Here we investigated a protein containing a CARF domain fused Toll/interleukin-1 receptor (TIR) domain, Cat1. We found that Cat1 provides immunity by cleaving and depleting NAD+ molecules from the infected host, inducing a growth arrest that prevents viral propagation. Cat1 forms dimers that stack upon each other to generate long filaments that are maintained by bound cOA ligands, with stacked TIR domains forming the NAD+ cleavage catalytic sites. Further, Cat1 filaments assemble into unique trigonal and pentagonal networks that enhance NAD+ degradation.

To understand the effects of Cat1 filamentation on the catalysis of NAD+ cleavage at the atomic level, we solved cryo-EM structures of cA4-bound Cat1 in the presence of a non-hydrolysable NAD+ analogue, benzamide adenine dinucleotide (BAD) or NAD+ at 3.3 Å and 4 Å resolution, respectively. We could resolve similar pentameric filament network formation for class 1 that represented the largest number of particles for both cA4-BAD-Cat1-His6 and cA4-NAD+-Cat1-His6 and therefore these were processed further, to the exclusion of other classes in both complexes that were part of the same network. We modelled a pair of Cat1 dimers in the map for each structure. In the case of the cA4− NAD+-Cat1-His6 structure, the observed density was sufficient to model ADPR, but neither the NAD+ substrate nor the other reaction product, NAM. In both cases we observed that residues S7, H8, N9, N10, D33, S68 and E74 from one TIR domain, and K121 and Y122 from the other, line the NADase active site. The BB-loop is predicted to control the access to the NADase active site in other TIR proteins. Both structures revealed that the active site is formed by two TIR domains from a pair of stacked Cat1 dimeric repeat units, suggesting that the catalytic activity relies on the multimerization of Cat1 dimers upon cA4 signal recognition. We tested the importance of these residues for Cat1 activity by making alanine substitutions (N10A, D33A, S68A, E74A, K121A and Y122A). The mutants were tested in vivo by measuring their toxicity during the type III-A CRISPR-Cas response and were all found to be defective in causing a growth arrest in staphylococci. While the D33A substitution reduced activity only partially, the Y122A mutation completely abrogated NAD+ cleavage. Altogether these data showed that Cat1 active site is formed through the interaction of two stacked TIR domains from different dimers, a finding that provides an explanation for the importance of filamentation for its enzymatic activity, as well as for the cooperativity of NAD+ cleavage.

>[4x]MPQAFFSHNNKDKKIVLEVLEHLRQSLVATWIDQQSIPGGGSLIQQIIAGISKSQYFLAFLSNEYLKSDWCWDELEQAYALHQKGKVKIIPILLTNRAQLDLNALTDARRNFLESILTRLKYVEFDPHNMTRSLGSVAEALWQNEAVRFEPIRMIKVNGTELQVVEFKIPGSNLPVDFLHHWDLKIEDFIATSPNEQKPVKFDVPVALYGPGPNWLYAFLTLPFKNRNTVFVFNSRTSEYICVYSKSAGLAPGMVLKGHHHHH> MNGWNFQELKETPSQTGGPYVHIGLLPKQANIEVFEHNLDNNLVQDNTQGQRIRLEGQVFDGLSLPLRDVLIE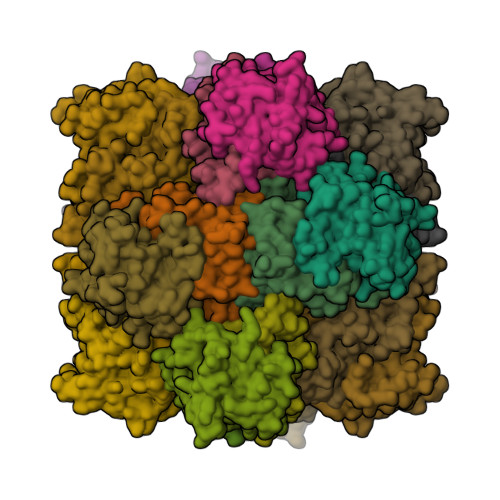IWQADTNGVYPSQADTQGKQVDPNFLGWGRTGADFGTGFWSFNTIKPGAVPGRKGSTQAPHISLIIFARGINIGLHTRVYFDDEAEANAKDPVLNSIEWATRRQTLVAKREERDGEVVYRFDIRIQGENETVFFDI;> MSQIIWGAYAQRNTEDHPPAYAPGYKTSVLRSPKNALISIAETLSEVTAPHFSADKFGPKDNDLILNYAKDGLPIGERVIVHGYVRDQFGRPVKNALVEVWQANASGRYRHPNDQYIGAMDPNFGGCGRMLTDDNGYYVFRTIKPGPYPWRNRINEWRPAHIHFSLIADGWAQRLISQFYFEGDTLIDSCPILKTIPSEQQRRALIALEDKSNFIEADSRCYRFDITLRGRRATYFENDLT2-amino-6-bromo-7-(trifluoromethyl)-1,8-naphthyridine-3-carboxamide 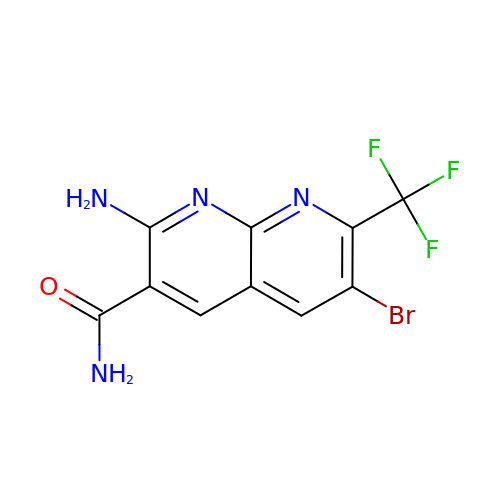| C10 H6 Br F3 N4 O | CENBBVPSOFGGNG-UHFFFAOYSA-N> GPGSMTNS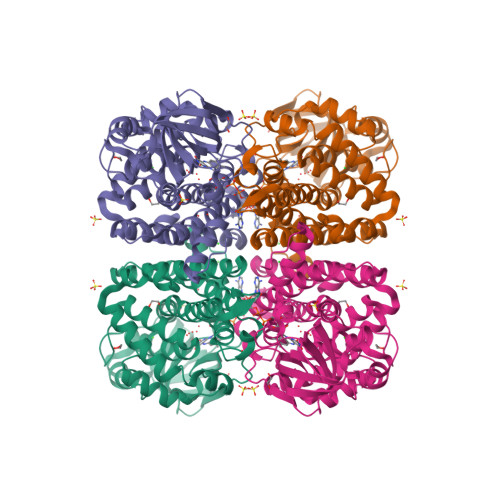AVAQPRSQRRGADDLIGINAVLSAEEREIRDTVRSVVQRRIKPHIASWYEDGELPARELAVELGELGLLGMHLKGYGCAGMSAVAYGLACLELEAGDSGIRSLVSVQGSLAMYAIHAFGSDEQKDQWLPDMASGHRIGCFGLTEPDHGSDPAGMRTRATRSGDDWILTGTKMWITNGSVADVAVVWARTDEGIRGFVVPTDTPGFTANTIKSKMSLRASVTSELVLDGVRLPDSARLPGATSLGAPLRCLNEARFGIVFGALGAARDCLETALAYACSREQFDRPIGGFQLTQQKLADMTLEYGKGFLLALHLGRQKDAGELAPEQVSLGKLNNVREAIEIARTARTVLGASGITGEYPVMRHANNLESVLTYEGTSEMHTLIIGQALTGVGAFR>SNADQKSRLVEEKRRAAKLAATLVEPDQTLFFDCGTTTPWIIEAIDNEIPFTAVCYSLNTFLALKEKPHCRAFLCGGEFHASNAIFKPIDFQQTLNNFCPDIAFYSAAGVHVSKGATCFNLEELPVKHWAMSMAQKHVLVVDHSKFGKVRPARMGDLKRFDIVVSDCCPEDEYVKYAQ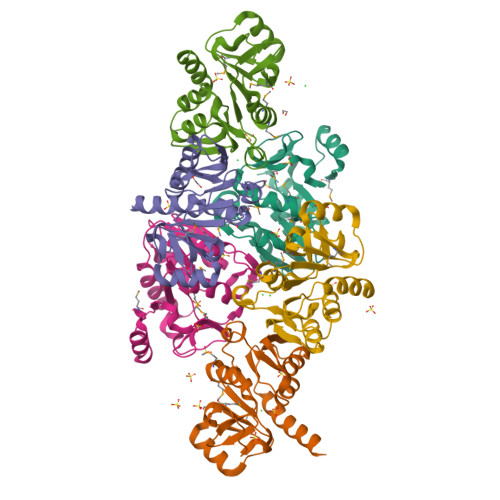TQRIKLMY[6x]> APLAHCDGRGGLKLSQDMDTCEDILPCVPFSVAKSVKSLYLGRMFSGTPVIRLRFKRLQPTRLVAEFDFRTFDPEGILLFAGGHQDSTWIVLALRAGRLELQLRYNGVGRVTSSGPVINHGMWQTISVEELARNLVIKVNRDAVMKIAVAGDLFQPERGLYHLNLTVGGIPFHEKDLVQPINPRLDGCMRSWNWLNGEDTTIQETVKVNTRMQCFSVTERGSFYPGSGFAFYSLDYMRTPLDVGTESTWEVEVVAHIRPAADTGVLFALWAPDLRAVPLSVALVDYHSTKKLKKQLVVLAVEHTALALMEIKVCDGQEHVVTVSLRDGEATLEVDGTRGQSEVSAAQLQERLAVLERHLRSPVLTFAGGLPDVPVTSAPVTAFYRGCMTLEVNRRLLDLDEAAYKHSDITAHS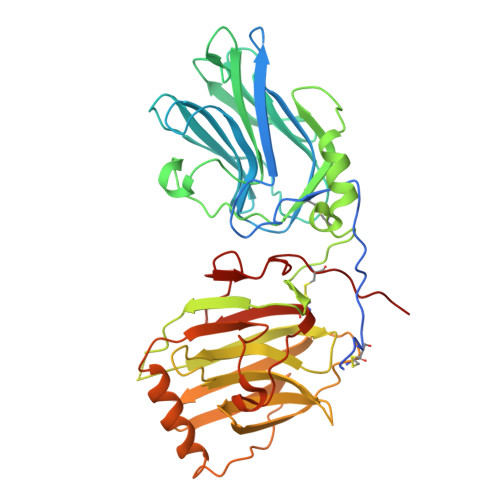CPPVEPAAA>GSHMLVEDKEDEVADLKQDTESLQKQLEENQEELEIVGNMLREEQGKVDQLQKRNVAHQK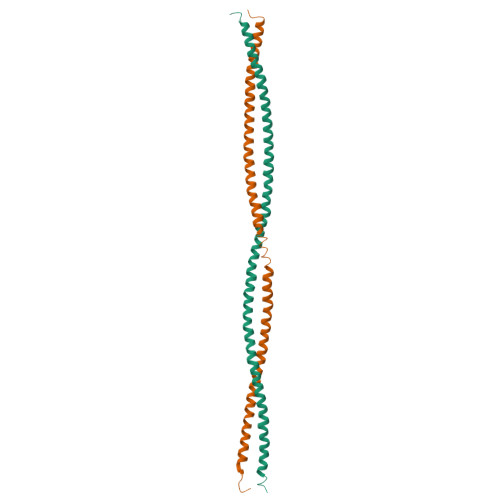EIGKLRAELGTAQRNLEKADQLLKRNSQQQNQQSLDMRKLGELEADLKEKDSMVESLTETIGILRKELENEKLKAAENMDSFEKLSMENENLKEKIAHYRAQRFSPA[2x]>GCATGCT[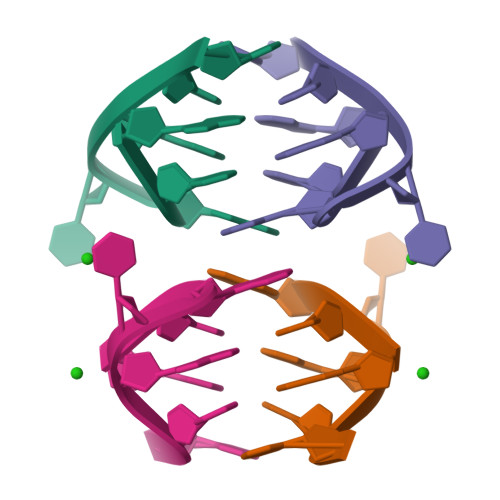2x]> MDPMICLGLEGTAEKTGVGIVTSDGEVLFNKTIMYKPPKQGINPREAADHHAETFPKLIKEAFEVVDKNEIDLIAFSQGPGLGPSLRVTATVARTLSLTLKKPIIGVNHCIAHIEIGKLTTEAEDPLTLYVSGGNTQVIAYVSKKYRVFGETLDIAVGNCLDQFARYVNLPHPGGPYIEELARKGKKLVDLPYTVKGMDIAFSGLLTAAMRAYDAGERLEDICYSLQEYAFSMLTEITERALAHTNKGEVMLVGGVAANNRLREMLKAMCEGQNVDFYVPPKEFCGDNGAMIAWLGLLM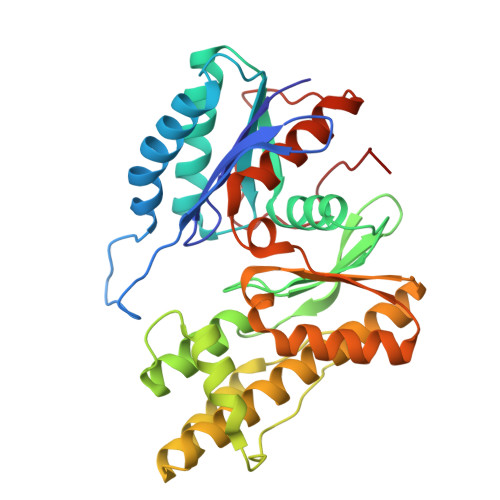HKNGRWMSLDETKIIPNYRTDMVEVNWI> GPHNMATLTDRTYLPPLEDCLTGRTVILSWRLVASALEDADLARLTSPALSTFLRDGFVHELLKHPARVFEPKDLKQEFETKTSSIQTVAPGVDTIKKDALWLADAVAINQVAALRIVLIEYQTRAHSHLVLPLSTQDVANIQEAAGVGDAHASSILSLLNPASAVDAETMWCDFETEARRRERILATYLSERRSFTAAVDALVTFLLHSAPGQHKDLDSLRRALLKDAFAFDEDLDVPDRSKLLTMAPTYMNLVEDCIARAQALPAKLGESFKTEAFELDWLRTAITEAVHSLSIAFQALDLDTPYFAPHELLSEWFELMNSSLFLESILGFEVVADLAMPARSLVSAICLKMLNIDRTIQFLHDFDYPDGEEPYLLSSQTLNKIHTAVTNAVNSGVAASLPVAFAWSLIVHQMHLGYQERAERRDLLVNQRAQAGFELEFQPSASTPNRRRRNSAGSIVSLEASPYDDFLREQRLDNDIAPVEQIAMLATSRGQVYQVMSEMALCLGTTHEAAFRPAVGARARLVFQDLLKRSAYLIPYQDEPVFSLLAILATGRQYWDVTDALSASSLNQVYTDMLDDETLFTQFTMQAINRFPYEFNPFSVLCRVLAAALITNKDKADVVTGWLWRTPTLTVDWNPAWDRSYELCFEDENTNSFRLTRDVDLFGSASPARPRHLAAEERFIIPEGTLGRFVTDVGRTARLEFEHSALALLGKRLEVKAAEEICDSGMAPLDVDEQAEAVAMLATVLRAESLKSTAKGGDPEAPLKFLKEASRLLPHNKDILTVISDTIDGLVEKELLELDGPQIAVLASCLQFLHAALAVCPGRVWAYMSRCALIAGDARPGRLSRITGSLDMYAERFDLLSSAVKLFAALIDSAACSAVQRRAGSTALVSVRSAVENPWLGTSEKILSRVALAIAQAALDVYESTTTWRFRSELDRSILVRDVVGLMHKLVVHAHTLSSHLTSTLSPAAAHIISSFLTPPPSASSLRFQPLLGTLLVALITPRATLYPGQSRILAERVTSVLAFCTSLLRAADFLGQTHIPLQTHLFQSACLLARLPAANAVYRAPVLELLRALVEVAGRAANGSGEPPSLLGYLGSHAARSFISLVEGIDKPFGRVEHAVVTWRFFAAVIRNRQQWMAGCLLTGRTPREALKGGGEQKIERKVGEGSVLAAAMERLREVKSLDVQEAVAVMDFVVSAQNYWPWTIFAVRKEKEVVDALRGYVRGLKAPGMVMKTDGAAAAAFQARIAAYVAETFAMQLYHMRQMRQAEKFAGELVADLDYFLREGVMVWGYNASLHGNFARNFAKRFPGVEVDDFKRTMWLPRELGKGYYYALEVAEQMLGFDAGWGGVKQSGFRKEMETANLNLSLVEAQVSLFHAWEYLLLELTLSLLPKKENAAFARQVLQVVEQCLEANQRSQPPENIFVVLGHARAGLALTLLQRLADANQLPRDVTHLLALVSSAIHAVENPFGANDLPYFRTLLKILFVVLRAAKQGTAKPGESNVAITQQVLTILDRVVARCFRALAALVHEQQQNATDGTTTAPEDLALITAILQACLSVPGIEQCQVQVLNIMAAHDVFQVAVALFSWADRLLPANPSPASSSTSTSATNPASGDPVYGELALLFLLELSALPALAEHLACDGLLGHLAAARLAGYMRRTNVGPFAENAGAARCYAIWAKCLLPLLLNILAALGSTVAPEVAWVLNQFPNLLQSSV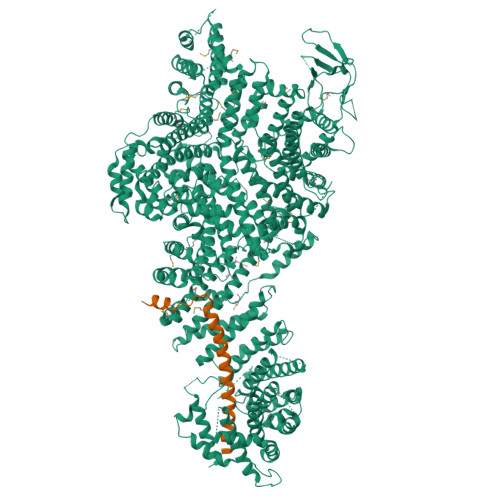ERIEPPGFSRPTLSLASTPPRQKFISLLEISEIHSLALLTRVLAACRAQNARDVPEVTWDGAKVLECVEYWLRGRKVLRERLVPLGPREVEWRGMVATGGVVGVAGDGGEGCENRLEEKAVGLLVGVREVLEGGLEGEGE;> SGTGLGEVDVDTYLSNLQTKTTLSMIADGLERSARDFDAFLEENVTLEWEAQRKRIYQHFGIK>[2x]MGFLAATLVSCAALASAASIPRPHAKRQVSQLRDDYDFVIVGGGTSGLTVADRLTEAFPAKNVLVIEYGDVHYAPGTFDPPTDWITPQPDAPPSWSFNSLPNPDMANTTAFVLAGQVVGGSSAVNGMFFDRASRHDYDAWTAVGGSGFEQSSHKWDWEGLFPFFQKSVTFTEPPADIVQKYHYTWDLSAYGNGSTPIYSSYPVFQWADQPLLNQAWQEMGIN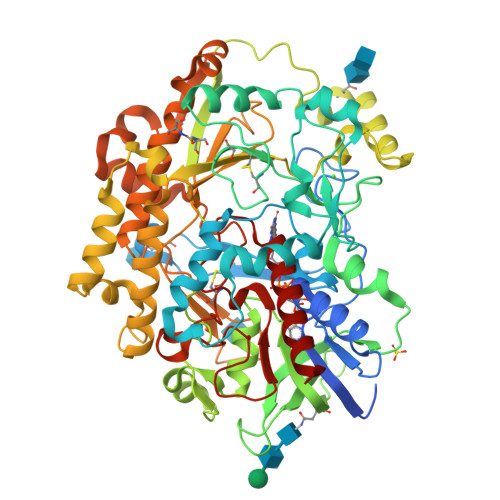PVTECAGGDKEGVCWVPASQHPVTARRSHAGLGHYADVLPRANYDLLVQHQVVRVVFPNGPSHGPPLVEARSLADNHLFNVTVKGEVIISAGALHTPTVLQRSGIGPASFLDDAGIPVTLDLPGVGANLQDHCGPPVTWNYTEPYTGFFPLPSEMVNNATFKAEAITGFDEVPARGPYTLAGGNNAIFVSLPHLTADYGAITAKIRAMVADGTAASYLAADVRTIPGMVAGYEAQLLVLADLLDNPEAPSLETPWATSEAPQTSSVLAFLLHPLSRGSVRLNLSDPLAQPVLDYRSGSNPVDIDLHLAHVRFLRGLLDTPTMQARGALETAPGSAVADSDEALGEYVRSHSTLSFMHPCCTAAMLPEDRGGVVGPDLKVHGAEGLRVVDMSVMPLLPGAHLSATAYAVGEKAADIIIQEWMDKEQ> VFHKIRNEDLIFNESLGQGTFTKFFKGVRREVGDYGQLHETEVLLKVLDKAHRNYSESFFEAASMMSKLSHKHLVLNYGVCVCGDENILVQEFVKFGSLDTYLKKNKNCI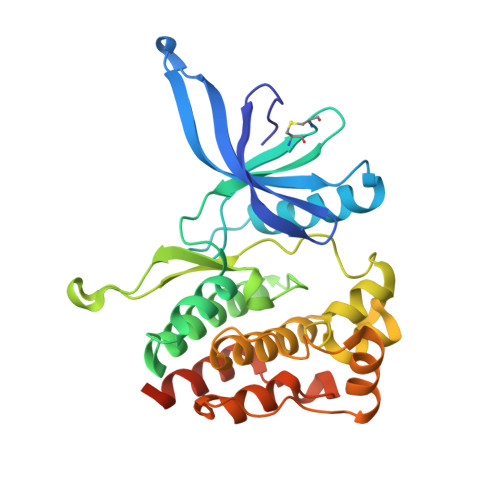NILWKLEVAKQLAAAMHFLEENTLIHGNVCAKNILLIREEDRKTGNPPFIKLSDPGISITVLPKDILQERIPWVPPECIENPKNLNLATDKWSFGTTLWEICSGGDKPLSALDSQRKLQFYEDRHQLPAPKAAELANLINNCMDYEPDHRPSFRAIIRDLNSLFTPDLVPRGSHHHHHH> KAVVPGPAEHPLQYNYTFWYSRRTPGRPTSSQSYEQNIKQIGTFASVEQFWRFYSHMVRPGDLTGHSDFHLFKEGIKPMWEDDANKNGGKWIIRLRKGLASRCWENLILAMLGEQFMVGEEICGAVVSVRFQEDIISIWNKTASDQATTARIRDTLRRVLNLPPNTIMEYKTHTDSIKMPGRLGPQRLLF;> GG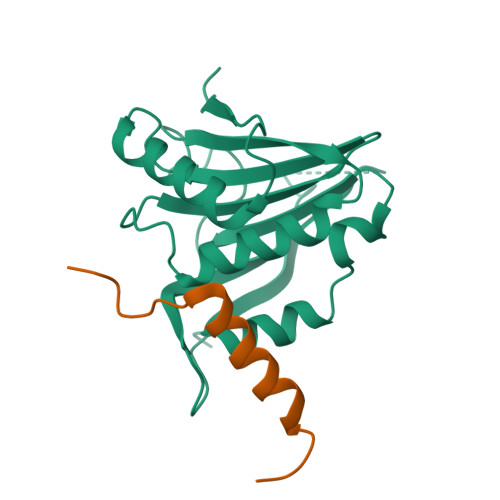KKKNKEGSGDGGRAELNPWPEYIYTRLEMYNILKAEHDSILAE> MKEFYLTVEQIGDSIFERYIDSNGRERTREVEYKPSLFAHCPESQATKYFDIYGKPCTRKLFANMRDASQWIKRMEDIGLEALGMDDFKLAYLSDTYNYEIKYDHTKIRVANFDIEVTSPDGFPEPSQAKHPIDAITHYDSIDDRFYVFDLLNSPYGNVEEWSIEIAAKLQEQGGDEVPSEIIDKIIYMPFDNEKELLMEYLNFWQQKTPVILTGWNVESFAIPYVYNRIKNIFGESTAKRLSPHRKTRVKVIENMYGSREIITLFGISVLDYIDLYKKFSFTNQPSYSLDYISEFELNVGKLKYDGPISKLRESNHQRYISYNIIAVYRVLQIDAKRQFINLSLDMGYYAKIQIQSVFSPIKTWDAIIFNSLKEQNKVIPQGRSHPVQPYPGAFVKEPIPNRYKYVMSFDLTSLYPSIIRQVNISPETIAGTFKVAPLHDYINAVAERPSDVYSCSPNGMMYYKDRDGVVPTEITKVFNQRKEHKGYMLAAQRNGEIIKEALHNPNLSVDEPLDVDYRFDFSDEIKE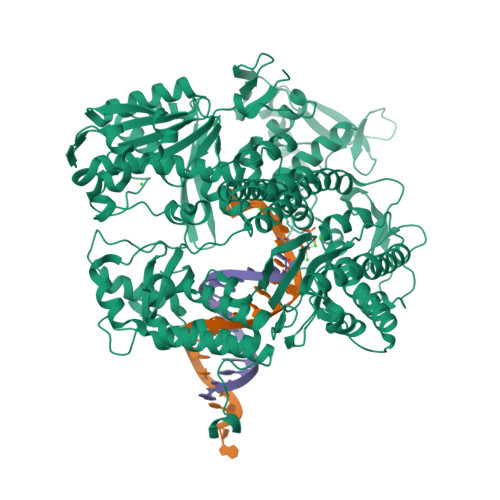KIKKLSAKSLNEMLFRAQRTEVAGMTAQINRKALINGLAGALGNVWFRYYDLRNATAITTFGQMALQWIERKVNEYLNEVCGTEGEAFVLYGDTDSIYVSADKIIDKVGESKFRDTNHWVDFLDKFARERMEPAIDRGFREMCEYMNNKQHLMFMDREAIAGPPLGSKGIGGFWTGKKRYALNVWDMEGTRYAEPKLKIMGLETQKSSTPKAVQKALKECIRRMLQEGEESLQEYFKEFEKEFRQLNYISIASVSSANNIAKYDVGGFPGPKCPFHIRGILTYNRAIKGNIDAPQVVEGEKVYVLPLREGNPFGDKCIAWPSGTEITDLIKDDVLHWMDYTVLLEKTFIKPLEGFTSAAKLDYEKKASLFDMFDF3-[3-(methylsulfonylaminomethyl)phenyl]benzoic acid | C15 H15 N O4 S | 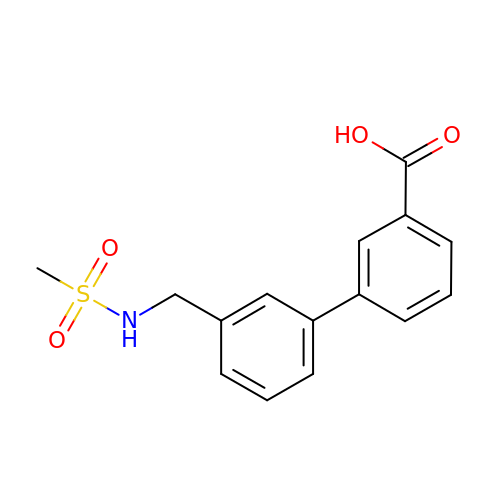SPDMRDWNPIVNCJ-UHFFFAOYSA-N The N protein is the most abundant viral protein in the Phlebovirus virion and plays a key role in encasing vRNA in a protective coat. In addition to its critical role in protecting the vRNA and the antigenome (cRNA), the N protein also plays an active role in RNA transcription and replication, as well as in virion assembly. Here, we present the crystal structure of RVFV N forming a hexameric ring. In conclusion, the structure of the hexamer formed by the RVFV N protein presented here shows that oligomerization is mediated by a flexible N-terminal arm, which binds a hydrophobic pocket in the adjacent subunit.

Using the N2 fraction, crystals were obtained in the P6 space group with unit cell parameters of a = b = 180.9 Å and c = 47.4 Å. *Values in parentheses give the values in the highest resolution shell (1.69–1.6 Å ). The six copies of subunit α that surround the crystallographic 6-fold symmetry axis (black dot) form one hexamer (labeled I), and the three βγ dimers that surround the crystallographic 3-fold symmetry axis (grey dot) form a second hexamer (labeled II). Hexamers I and II face in opposite directions and are offset by approximately 10 Å in the direction of the c axis. Hexamers I and II in the crystals of the native protein superimpose very well, but the two rings in the crystals of the selenomethionyl protein are slightly different. We have determined the crystal structure of RVFV N in a hexameric form, which shows largely the same fold that was previously seen in a crystal structure of monomeric N. The two structures differ, however, in the position of the N-terminal arm. In the previous structure, the N-terminal arm packs closely against the core domain, while it extends away from it in our structure. Extension of the N-terminal arm is crucial for the oligomerization of N, as it mediates the interaction with the adjacent subunit in the crystallographic hexamer. (D) Docking of the crystal structure of hexamer I formed by native N into the EM density map of the hexameric N-RNA complex.

>MDNYQELRVQFAAQAVDRNEIEQWVREFAYQGFDARRVIELLKQYGGADWEKDAKKMIVLALTRGNKPRRMMMKMSKEGKATVEALINKYKLKEGNPSRDELTLSRVAAALAGWTCQALVVLSEWLPVTGTTMDGLSPAYPRHMMHPSFAGMVDPSLPGDYLRAILDAHSLYLLQFSRVINPNLRGRTKEEVAATFTQPMNAAVNSNFISHEKRREFLKAFGLVDSNGKPSAAVMAAAQAYKTAA[3x]>PRGSHGQQCRSRFVKKDGHCNVQFINVGEKRNETLVFSHNAVIAMRDGKLCLMWRVGNLRKSHLVEAHVRAQLLKSRITSEGEYIPLDQIDINVGFDSGIDRIFLVSPITIVHEIDEDSPLYDLSKQDIDNADFEIVVILEGMVEATAMTTQCRSSYLANEILWGHRYEPVLFEEKH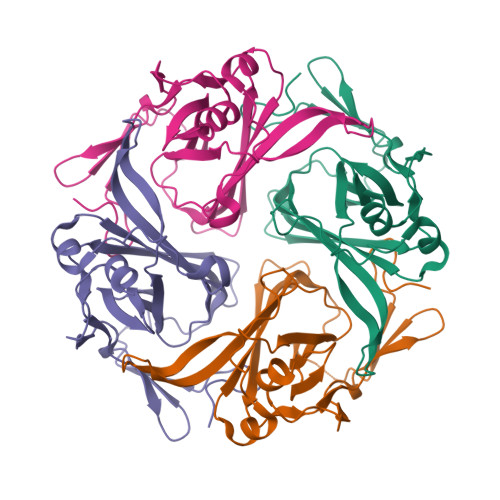YYKVDYSRFHKTYEVPNTPLCSARDLAEKKYILSNANSFCYENEVALTSKEEEEDSENGVPESTSTDSPPGIDLHNQASVPLEPRPLRRESEI[4x]>MRMVDLIAKKRDGKALTKEEIEWIVRGYTNGDIPDYQMSALAMAIYFRGMTEEETAALTMAMVQSGEMLDLSSIRGVKVDKHSTGGVGDTTTLVLGPLVASVGVPVAKMSGRGLGHTGGTIDKLESVPGFHVEISKDEFIRLVNENGIAIIGQTGDLTPADKKLYALRDVTATVNSIPLIASSIMSKKIAAGADAIVLDVKTGAGAFMKKLDEARRLARVMVDIGKRVGRRTMAVISDMSQPLGYAVGNALEVKEAIETLKGNGPHDLTELCLTLGSHMVYLAEKAPSLDEARRLLEEAIRSGAAIAAFKTFLAAQGGDASVVDDLDKLPKAAYTSTV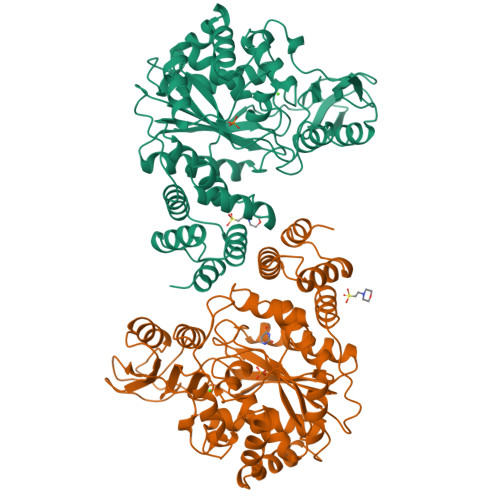TAAADGYVAEMAADDIGTAAMWLGAGRAKKEDVIDLAVGIVLHKKIGDRVQKGEALATIHSNRPDVLDVKEKIEAAIRLSPQPVARPPLIYETIV[2x]>MANSPVSVFGLGAMGTALATQFLRKGHKTTVWNRTPAKAQPLIAIGASHAPTIDSAAAASSLLIICQLDKASVMQTLQQAPTAWAAKTIVDLTNGTPAHARETADWALAHGARYIHGGIMAVPFMIGQPDAMILYSGPAEVFEGVKDTLSVLGTNTYVGEDVGLASLHDLALLSGMYGLFSGFTHAVALVQSANIPAAGFVATQLIPWLTAMTQHLNLLATQVDEKDYGDGGSSLDMQAKAAPNILEASQAQGVSVELIQPIFKLIERRVEEGKGSEGLAALVGMIMK[2x]

The NADPH-dependent imine reductase from Ajellomyces dermatitidis (AdRedAm) catalyzes the reductive amination of certain ketones with amine donors supplied in an equimolar ratio. The two AdRedAm monomers associate to form a dimer in which reciprocal domain sharing results in the formation of a large active-site cleft between the N-terminal domain of one monomer and the C-terminal domain of its partner. One of them, AdRedAm from Ajellomyces dermatitidis, has been reported to be more stable than AspRedAm and thus perhaps more suitable for process applications.

The first form, which belongs to space group P3121 and was refined to 2.01 Å resolution, features two molecules (one dimer) in the asymmetric unit in complex with the redox-inactive cofactor NADPH4. Using data set 1, the structure of AdRedAm was solved using the structure of AspRedAm (sequence identity of 54%) as a model. The structure was built and refined using iterative cycles of building in Coot and refinement in REFMAC. This data set yielded two molecules in the asymmetric unit as a dimer, which is the canonical form of previously described imine reductases. Electron density for the backbone atoms was largely complete throughout the length of both chains from Ala2 to Lys288. Interestingly, the other active site featured no cofactor density. A comparison of monomers with and without NADPH4 showed that the side chain of Asn94 was rotated approximately 180° to accommodate the ribose of the cofactor, but that the orientation of the other side chains was largely conserved. The AdRedAm dimer observed in the structure from data set 1 was already instructive in showing two possible states of the monomer in which the non-natural cofactor molecule was either absent or bound.ABCC4 (ATP-binding cassette sub-family C member 4) is a transporter protein that is primarily localized to the plasma membrane, and its efflux activity is associated with the progression of various cancers and the development of drug resistance. The ABCC4 protein primarily consists of four domains, namely, two transmembrane domains (TMDs) and two nucleotide-binding domains (NBDs). Structurally distinct from other C-family proteins, ABCC4 lacks a TMD0 domain. ABCC4 can transport a diverse range of substrates, and its involvement in numerous vital cellular physiological processes has been well documented.

The hABCC4-Apo structure was used to illustrate the substrate-binding pocket of hABCC4 and the state of the pocket in the absence of substrate binding. On the basis of the analytical structural data, the resolved hABCC4 protein exhibited an average resolution of 3.29 Å. Comparison of the density maps of the substrate-binding pocket between hABCC4 (Apo) and the other three complex structures clearly reveals the density of the substrate molecules within the binding pocket in the three complex structures. These structures (Fig. 2 right side cartoon) revealed that the substrate-binding region of hABCC4 is a cavity formed by helices TM2, TM3, TM5, and TM6 in the TMD1 domain and helices TM9, TM11, and TM12 in the TMD2 domain. Helices TM2, TM3, TM5, TM6, TM9, and TM11 collectively form an approximately elliptical cavity surrounding the periphery, whereas helix TM12 traverses the central axis of the cavity. In the top-down view, the binding region appears as a fan-shaped pocket. The outer ring of the pocket is surrounded by residues F156, F211, F324, L363, L367, F368, and R946, whereas the center of the pocket contains residues Q994, W995, and R998 located in helix TM12.

> MLPVYQEVKPNPLQDANLCSRVFFWWLNPLFKIGHKRRLEEDDMYSVLPEDRSQHLGEELQGFWDKEVLRAENDAQKPSLTRAIIKCYWKSYLVLGIFTLIEESAKVIQPIFLGKIINYFENYDPMDSVALNTAYAYATVLTFCTLILAILHHLYFYHVQCAGMRLRVAMCHMIYRKALRLSNMAMGKTTTGQIVNLLSNDVNKFDQVTVFLHFLWAGPLQAIAVTALLWMEIGISCLAGMAVLIILLPLQSCFGKLFSSLRSKTATFTDARIRTMNEVITGIRIIKMYAWEKSFSNLITNLRKKEISKILRSSCLRGMNLASFFSASKIIVFVTFTTYVLLGSVITASRVFVAVTLYGAVRLTVTLFFPSAIERVSEAIVSIRRIQTFLLLDEISQRNRQLPSDGKKMVHVQDFTAFWDKASETPTLQGLSFTVRPGELLAVVGPVGAGKSSLLSAVLGELAPSHGLVSVHGRIAYVSQQPWVFSGTLRSNILFGKKYEKERYEKVIKACALKKDLQLLEDGDLTVIGDRGTTLSGGQKARVNLARAVYQDADIYLLDDPLSAVDAEVSRHLFELCICQILHEKITILVTHQLQYLKAASQILILKDGKMVQKGTYTEFLKSGIDFGSLLKKDNEESEQPPVPGTPTLRNRTFSESSVWSQQSSRPSLKDGALESQDTENVPVTLSEENRSEGKVGFQAYKNYFRAGAHWIVFIFLILLNTAAQVAYVLQDWWLSYWANKQSMLNVTVNGGGNVTEKLDLNWYLGIYSGLTVATVLFGIARSLLVFYVLVNSSQTLHNKMFESILKAPVLFFDRNPIGRILNRFSKDIGHLDDLLPLTFLDFIQTLLQVVGVVSVAVAVIPWIAIPLVPLGIIFIFLRRYFLETSRDVKRLESTTRSPVFSHLSSSLQGLWTIRAYKAEERCQELFDAHQDLHSEAWFLFLTTSRWFAVRLDAICAMFVIIVAFGSLILAKTLDAGQVGLALSYALTLMGMFQWCVRQSAEVENMMISVERVIEYTDLEKEAPWEYQKRPPPAWPHEGVIIFDNVNFMYSPGGPLVLKHLTALIKSQEKVGIVGRTGAGKSSLISALFRLSEPEGKIWIDKILTTEIGLHDLRKKMSIIPQEPVLFTGTMRKNLDPFNEHTDEELWNALQEVQLKETIEDLPGKMDTELAESGSNFSVGQRQLVCLARAILRKNQILIIDEATANVDPRTDELIQKKIREKFAHCTVLTIAHRLNTIIDSDKIMVLDSGRLKEYDEPYVLLQNKESLFYKMVQQLGKAEAAALTETAKQVYFKRNYPHIGHTDHMVTNTSNGQPSTLTIFETAL> MLNKAEQISEKSERAYVERFVN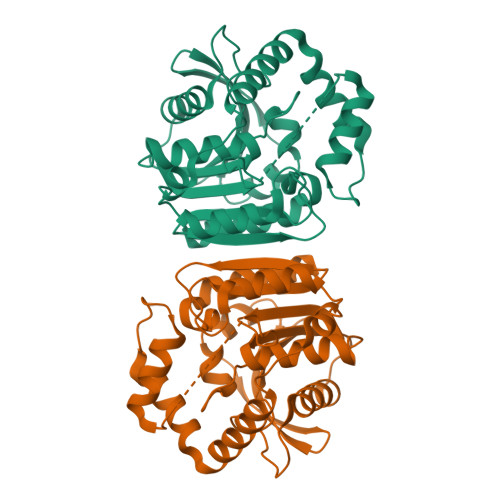AGGVETRYLEAGKGQPVILIHGGGAGAESEGNWRNVIPILARHYRVIAMDMLGFGKTAKPDIEYTQDRRIRHLHDFIKAMNFDGKVSIVGNSMGGATGLGVSVLHSELVNALVLMGSAGLVVEIHEDLRPIINYDFTREGMVHLVKALTNDGFKIDDAMINSRYTYATDEATRKAYVATMQWIREQGGLFYDPEFIRKVQVPTLVVQGKDDKVVPVETAYKFLDLIDDSWGYIIPHCGHWAMIEHPEDFANATLSFLSLRVDITPAAAHHHHHH Bub1 and BubR1 are paralogous proteins at the core of the SAC. Contrarily to BubR1, Bub1 is a bona fide kinase, but its activity is believed to play a marginal role in the SAC. Bub1 phosphorylates Thr120 of histone H2A (P-T120-H2A), which in turn promotes centromere accumulation of Shugoshin and protein phosphatase 2A (PP2A), thus contributing to the establishment and protection of centromeric cohesion as well as to Aurora B kinase recruitment. Like other members of the eukaryotic protein kinase family, Bub1 consists of a small N-terminal lobe (N-lobe) rich in β-sheet structure, and a larger C-terminal lobe (C-lobe) rich in α-helices.

When incubated with 1 mM ATP for 16 hours, Bub1kinase auto-phosphorylates. LC-MS/MS spectra demonstrated S969 to be the only prominently phosphorylated residue in Bub1kinase (not shown), in agreement with a recent study. Our crystal structure of the phosphorylated kinase captured the P+1 loop in a conformation that creates a steric blockade to the active site, with the phosphate attached to the side chain of S969 pointing towards the nucleotide-binding pocket of Bub1. The phosphate group of pS969 points directly towards the co-crystallized ADP molecule, positioning the P+1 loop in such a way that it would be expected to prevent the ingression of a substrate peptide. The position of the phosphate on P-S969 is very close to that expected for the γ-phosphate should ATP, instead of ADP, sit in the binding site. In this position, the phosphate faces a highly negatively charged environment created by the directly neighboring residues E967 and D917. Electrostatic repulsion would be expected to extrude the phosphorylated P+1 loop, possibly explaining the conformation demonstrated by the recently published structure of P-969-Bub1kinase. Thus, we suspect that the conformation we have trapped is stabilized by contacts with symmetry mates in the crystal. It provides what appears to be an intermediate conformation of the P+1 loop after phosphate transfer, before extrusion from the active site. Collectively, the three structures likely depict Bub1 at different stages of the auto-phosphorylation process, and are consistent with the idea that phosphorylation at P-S969 is required to remove a steric blockade of the active site by the P+1 loop.

>[2x]GPMDPSSLGTVDAPNFIVGNPWDDKLIFKLLSGLSKPVSSYPNTFEWQCKLPAIKPKTEFQLGSKLVYVHHLLGEGAFAQVYEATQGDLNDAKNKQKFVLKVQKPANPWEFYIGTQLMERLKPSMQHMFMKFYSAHLFQNGSVLVGELYSYGTLLNAINLYKNTPEKVMPQGLVISFAMRMLYMIEQVHDCEIIHGDIKPDNFILGNGFLEQDDEDDLSAGLALIDLGQSIDMKLFPKGTIFTAKCETSGFQCVEMLSNKPWNYQIDYFGVAATVYCMLFGTYMKVKNEGGECKPEGLFRRLPHLDMWNEFFHVMLNIPDCHHLPSLDLLRQKLKKVFQQHYTNKIRALRNRLIVLLLECKRSRK> GPKDYDELLKYYE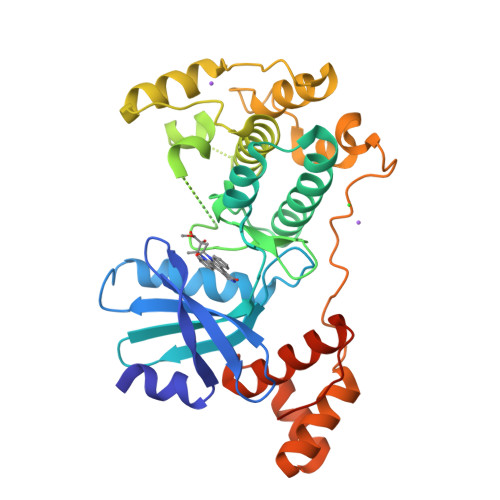LHETIGTGGFAKVKLACHILTGEMVAIKIMDKNTLGSDLPRIKTEIEALKNLRHQHICQLYHVLETANKIFMVLEYCPGGELFDYIISQDRLSEEETRVVFRQIVSAVAYVHSQGYAHRDLKPENLLFDEYHKLKLIDFGLCAKPKGNKDYHLQTCCGSLAYAAPELIQGKSYLGSEADVWSMGILLYVLMCGFLPFDDDNVMALYKKIMRGKYDVPKWLSPSSILLLQQMLQVDPKKRISMKNLLNHPWIMQDYNYPVEWQSKNPFIHLDDDCVTELSVHHRNNRQTMEDLISLWQYDHLTATYLLLLAKKARGKPVRLRLSSFSCGHHHHHH>[2x]MKFGNFLLTYQPPELSQTEVMKRLVNLGKASEGCGFDTVWLLEHHFTEFGLLGNPYVAAAHLLGATETLNVGTAAIVLPTAHPVRQAEDVNLLDQMSKGRFRFGICRGLYDKDFRVFGTDMDNSRALMDCWYDLMKEGFNEGYIAADNEHIKFPKIQLNPSAYTQGGAPVYVVAESASTTEWAAERGLPMILSWIINTHEKKAQLDLYNEVATEHGYDVTKIDHCLSYITSVDHDSNRAKDICRNFLGHWYDSYVNATKIFDDSDQTKGYDFNKGQWRDFVLKGHKDTNRRIDYSYEINPVGTPEECIAIIQQDIDATGIDNICCGFEANGSEEEIIASMKLFQSDVMPYLKEKQ;>MKFGLFFLNFMNSKRSSDQVIEEM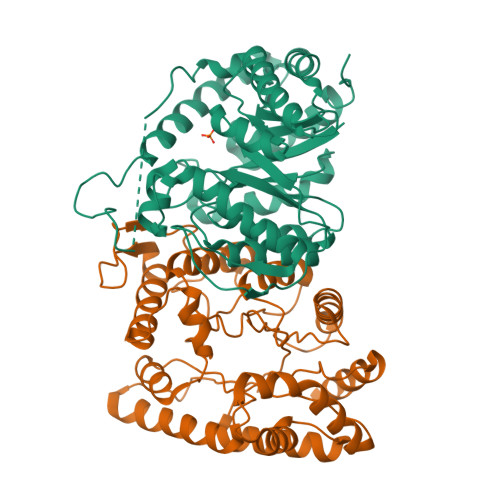LDTAHYVDQLKFDTLAVYENHFSNNGVVGAPLTVAGFLLGMTKNAKVASLNHVITTHHPVRVAEEACLLDQMSEGRFAFGFSDCEKSADMRFFNRPTDSQFQLFSECHKIINDAFTTGYCHPNNDFYSFPKISVNPHAFTEGGPAQFVNATSKEVVEWAAKLGLPLVFRWDDSNAQRKEYAGLYHEVAQAHGVDVSQVRHKLTLLVNQNVDGEAARAEARVYLEEFVRESYSNTDFEQKMGELLSENAIGTYEESTQAARVAIECCGAADLLMSFESMEDKAQQRAVIDVVNANIVKYHS[2x]>MAHHHHHHVDDDDKENLYFQGMVAEVQKQAPPFKKTAVVDGIFEEISLEKYKGKYVVLAFVPLAFSFVCPTEIVAFSDAAKKFEDQGAQVLFASTDSEYSLLAWTNLPRKDGGLGPVKVPLLADKNHSLSRDYGVLIEKEGIALRGLFIIDPKGIIRHITINDLSVGRNV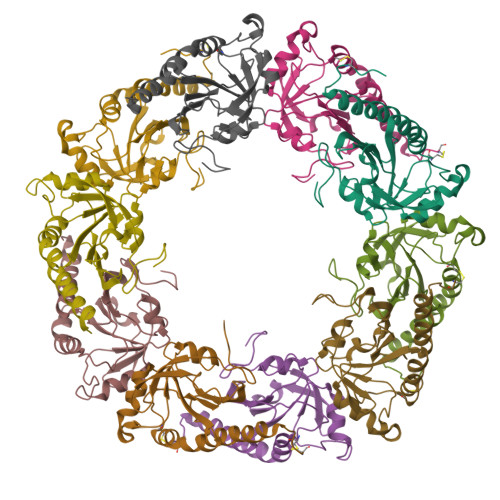NEALRLVEGFQWTDKNGTVLPCNWTPGAATIKPDVKDSKEYFKNANN[10x]> MSIVRIAPEINLVMDTESGTVTQERKDSIQYSMEPVFERVDKLDAIADDLVNSLSPSKPLLNTWPGRENTSYIAGIYSNSFYGIIVGLAFSGLLALIIYITRLMGGVV;> MAEEHEKGVPMVLAPQMGAIDATVESIRYRAQLIARNQKLDSGVAATGIIGFAAGFLFSLLMVIVLPVAVGL;>MFKFDKKQEVFELGGVKFGGQPGENPTVLVSTMFYARHKIVTDEDKGIFDRAAAETLWNTQVSLSDATGLPYVNQIVGETPESIKRYIEWFVGIDDRTPFLIDSSAGNVRAAAAQYCTEIGVADRAIHNSINASIEQSEIDVLTESDVSAAIVLAFNATDPTVKGKIDILEVGGSGQTKGMLQVAKECGIKYPIIDVAAMPLGAGSGATIRSVPTLKGKFGLPIGGGYHNMASAWDWLRKFKKTQPDPKAIYMPTDIGTNLVAQIAGSDYLLYGPIENVNQIFPAVAMVDIMLGETAKELGVEIADLEN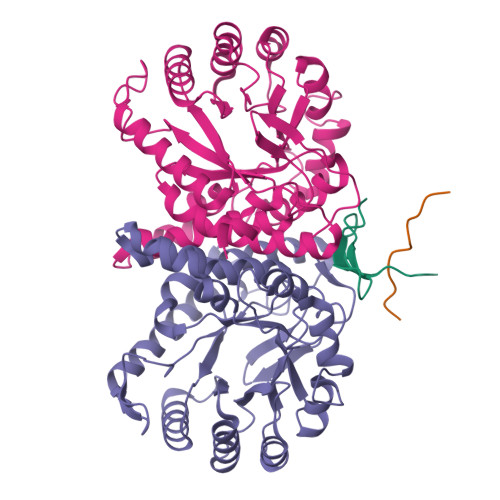HPVTKLT[2x]>[2x]MAQKDVLTDLSRVRNFGIMAHIDAGKTTTTERILYYTGINYKIGEVHDGAATMDWMEQEQERGITITSAATTTFWKDNQLNIIDTPGHVDFTVEVERNLRVLDGAVAVFDGKEGVEPQSEQVWRQADKYDVPRICFVNKMDKIGADFYFSVRTMGERLGANAVPIQLPVGAEADFEGVVDLVEMNAKVWRGETKLGETYDTVEIPADLAEQAEEYRTKLLEVVAESDEHLLEKYLGGEELTVDEIKGAIRKLTIASEIYPVLCGSAFKNKGVQPMLDAVVDYLPSPLDVPPAIGHAPAKEDEEVVRKATTDEPFAALAFKIATHPFFGKLTYIRVYSGTVESGSQVINATKGKKERLGKLFQMHSNKENPVDRASAGHIYAVIGLKDTTTGDTLSDPNQQIVLESMTFPDPVIEVAIEPKTKSDQEKLSLSIQKLAEEDPTFKVHLDSETGQTVIGGMGELHLDILVDRMRREFKVEANVGKPQVAYKETIKRLVQNVEY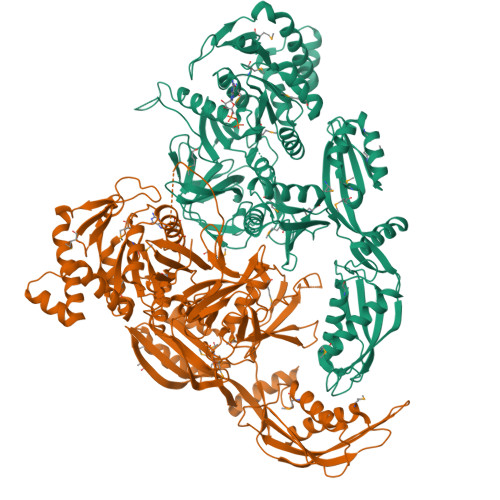THKKQTGGSGQFAKVIINLEPFTGEEGATYEFESKVTGGRIPREYIPSVDAGAQDAMQYGVLAGYPLVNLKVTLLDGAYHEVDSSEMAFKIAGSQVLKKAAALAQPVILEPIMAVEVTTPEDYMGDVIGDLNSRRGQIQAMEERAGARVVRAHVPLSEMFGYVGDLRSKTQGRANYSMVFDSYSEVPANVSKEIIAKATGELEGHHHHHH Recent studies revealed that protein phosphatase 4 (PP4), a ubiquitous and essential PPP, regulates a variety of cellular processes, including chromatin biology, DNA repair and cell cycle progression. The major form of PP4, conserved from yeast to human cells, comprises PP4c in complex with R2 and R3. Flfl14, the R3-type subunit of Drosophila PP4, has been shown to bind Miranda (Mira) and so recruits PP4 (PP4c–R2–R3Falafel) to regulate asymmetric division of neuroblasts. Here we show that Flfl directly binds the centromeric protein C (CENP-C) and brings PP4 activity to centromeres.

To better understand the molecular basis for the Flfl–CENP-C interaction, we co-crystallized an amino-terminal 122-aa-long fragment of Flfl containing the EVH1 domain (Flfl1–122) and the CENP-CFIM peptide and solved the structure by molecular replacement to 1.5 Å resolution as described in Methods. The final model comprises residues 4–114 of Flfl and 1055–1065 of CENP-C. We found that the Flfl1–122 fragment is composed of a seven-stranded β barrel capped by a C-terminal α-helix. Two concave surfaces are formed by the outside of each β sheet, one of which (strands β1, β2, β5, β6 and β7) forms the peptide-binding groove with contributions from an inter-strand loop (residues 66–69). The CENP-C peptide can be unambiguously identified as bound into that groove. The binding site lies in a highly conserved groove on the surface of the protein burying 1,700 Å2 of the total 6,700 Å2 surface of Flfl1–122 and corresponds to the surface responsible for binding proline-rich sequences in other members of the EVH1 family. Residues 1055–1065 of the CENP-CFIM peptide are well defined in the electron density, and include FKKP motif of the residues predicted to interact with the Flfl1–122 by peptide array analysis. The peptide backbone adopts a left-handed helical conformation similar to the polyproline II (PPII) helix28. This arrangement is mainly stabilized by the establishment of hydrogen bonding and van der Waals interaction between Pro1060 and Trp20. Additional residues flanking the PPII sequence provide directional specificity. In our structure CENP-C′s Phe1057 and Pro1060 provide the principle specificity and directionality of binding (see also the legend for Supplementary Fig. 2e). We suggest that Flfl–FIM interaction constitutes a novel mode of EVH1 binding in which a low proline content ligand is recognized in a PPII conformation.

> TTDTRRRVKLYALNAERQWDDRGTGHVSSTYVERLKGISLLVRAESDGSLLLESKIQPDTAYQKQQDTLIVWSEGDNFDLALSFQEKAGCDEIWEKICQVQGKDPSVEITQDIVEESEDERF;> PDESSADVVFKKPLAPAPR>GTGMESKYKEILLLTGLDNITDEELDRFKFFLSDEFNIATGKLHTANRIQVATLMIQNAGAVSAVMKTIRIFQKLNYMLLAKRLQEEKEKVDKQYKSVTKPKPLSQAEMSPAASAAIRND[21x]

AIM2 (absent in melanoma 2) is a bipartite protein composed of the N-terminal PYD followed by the dsDNA-binding HIN domain (hematopoietic interferon-inducible nuclear antigen). PYDs are six-helix bundles that belong to the death-domain (DD) superfamily and can assemble into helical filaments. The upstream PYD filaments then nucleate the filamentation of the PYD of central adaptor ASC (ASCPYD), leading to the oligomerization of the CARD of ASC (ASCCARD) to recruit and trigger the polymerization (activation) of procaspase-1 (ASC: apoptosis-associated speck-forming protein containing caspase-recruiting domain (CARD); CARDs are also six-helix bundles that belong to the DD family). AIM2 is essential for the host defense against numerous pathogenic viruses and bacteria.

Thus, we first determined the cryo-EM structure of the AIM2PYD filament using an untagged recombinant protein. Cryo-EM images showed that AIM2PYD filaments are straight helical rods. The average power spectrum of 512-pixel-long nonoverlapping filament segments showed that the AIM2PYD filament displays a six-start, C3 helical symmetry of 54.4° rotation (~6 subunits per helical turn) and an axial rise of 14 Å. These parameters are remarkably similar to those of the ASCPYD filament, further solidifying the concept that the upstream receptors provide structural templates for downstream assemblies in inflammasomes. The resolution of the final model was 3.2 Å according to the gold standard method. The diameter of the outer rim is ~94 Å and that of the inner cavity is ~25 Å. As seen from the ASCPYD filament, each AIM2PYD subunit contributes three unique protein–protein interaction interfaces. The type 1a:1b interface is largely composed of side-chain interactions, while the type 2a:2b and type 3a:3b interfaces involved both side-chain and backbone interactions. Aligning the new AIM2PYD filament to the GFP-AIM2PYD filament demonstrates that although the lateral interactions are largely conserved, the axial positions are significantly different due to the altered helical symmetry (five subunits per turn in the GFP-tagged filament vs. six subunits per turn in the untagged filament). On the other hand, aligning the cryo-EM structures of AIM2PYD and ASCPYD filaments demonstrates their congruent architectures.> GPHMSAFEEKAIEKVDDLLESYMGIRDTELAATMVELGKDKRNPDELA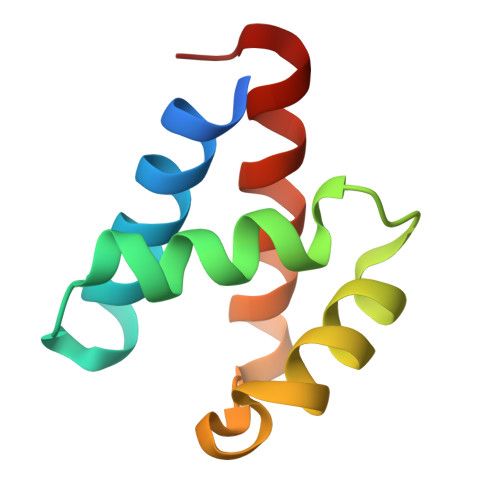EALDERLGDFAFPDEFVFDVWGAIGDAKVGRY> MDGSGEQPRGGGPTSSEQIMKTGALLLQGFIQDRAGRMGGEAPELALDPVPQDASTKKLSESLKRIGDELDSNMELQRMIAAVDT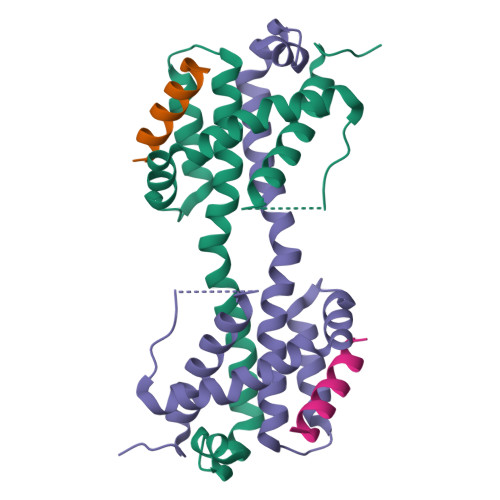DSPREVFFRVAADMFSDGNFNWGRVVALFYFASKLVLKALSTKVPELIRTIMGWTLDFLRERLLGWIQDQGGWDGLLSYGSS;> DMRPEIWIAQELRRIGDEFN>ADPALADVCRTKLPSQAQDTLALIAKNGPYPYNRDGVVFENRESRLPKKGNGYYHEFTVVTPGSNDRGTRRVVTGGYGEQYWSPDHYATFQ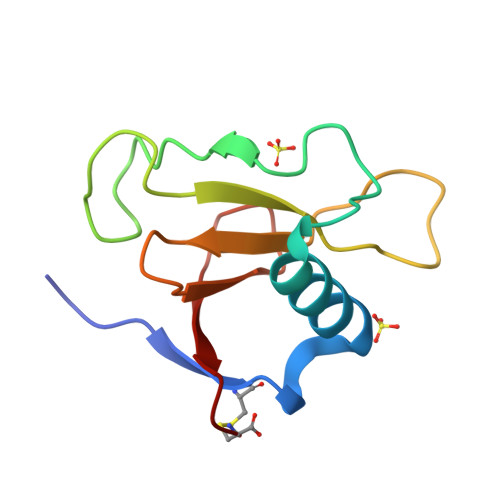EIDPRC[2x]> VGAITTIEDPVLAKKVPETFPELKPGESRHTSDHMSIYKFMGRSHFLCTFTFNSNNKEY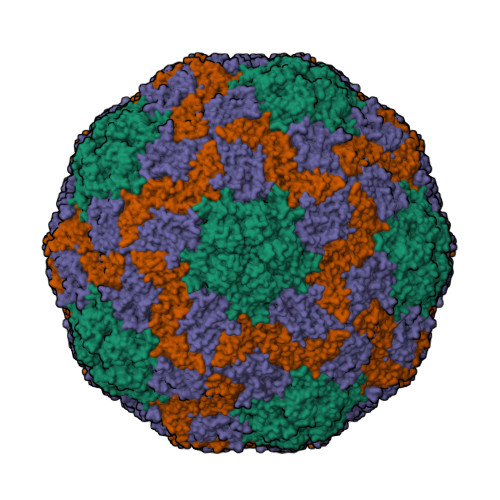TFPITLSSTSNPPHGLPSTLRWFFNLFQLYRGPLDLTIIITGATDVDGMAWFTPVGLAVDTPWVEKESALQIDYKTALGAVRFNTRRTGNIQIRLPWYSYLYAVSGALDGLGDKTDSTFGLVSIQIANYNHSDEYLSFSCYLSVTEQSEFYFPRAPLNSNAMLST;> ASYFTSVDQSSVHTAEVGSHQIEPLKTSVDKPGSKKTQGEKFFLIHSARWLTTHALFHEVAKLDVVKLLYNEQFAVQGLLRYHTYARFGIEIQVQINPTPFQQGGLICAMVPGDQSYGSIASLTVYPHGLLNCNINNVVRIKVPFIYTRGAYHFKDPQYPVWELTIRVWSELNIGTGTSAYTSLNVLARFTDLELHGLTPLST;> MMRNETRVSTTENVVNLSNYEDARAKMSFALDQEDWKSDPSQGGGIKITHFTTWTSIPTLAAQFPFNASDSVGQQIKVIPVDPYFFQMTNTNPDQKCITALASICQMFCFWRGDLVFDFQVFPTKYHSGRLLFCFVPGNELIDVTGITLKQATTAPCAVMDIAGVQSTLRFRVPWISDTPYRVNRYTKEAHQKGEYTAIGKLIVYCYNRLTSPSNVAHHVRVNVYLSAINLECFAPLYHAMDVTTQ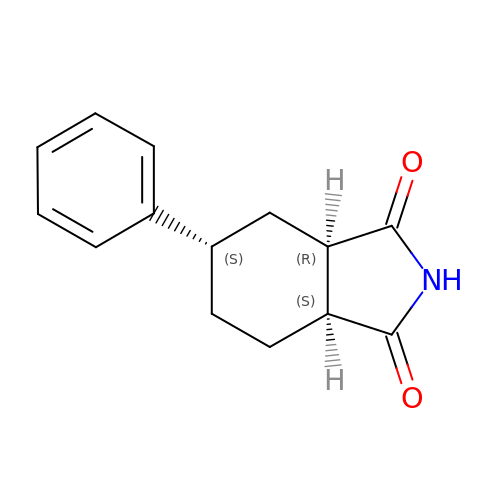(3~{a}~{R},5~{S},7~{a}~{S})-5-phenyl-3~{a},4,5,6,7,7~{a}-hexahydroisoindole-1,3-dione | C14 H15 N O2 | SHLALXCFPAKZHG-SDDRHHMPSA-N An understudied class of proteins in phosphotyrosine signaling, the receptor protein tyrosine phosphatases (RPTPs), are a family of single-pass transmembrane proteins whose architecture include an extracellular domain resembling those of cell adhesion molecules (CAMs) and intracellular single or tandem tyrosine phosphatase domains. In vertebrates, this diversity is typified by the leukocyte common antigen related (Lar) and its two homologs RPTPδ/PTPRD and RPTPσ/PTPRS, which form the type IIa family of RPTPs. The ectodomains of Lar-RPTPs resemble immunoglobulin (Ig)-superfamily CAMs and include three Ig-like domains followed by four to nine fibronectin type III (FN) repeats. Surprisingly, we uncovered a tripeptide, Lys-Gly-Asp (KGD), in the Dlar FN5 domain that is similar to the RGD motif in FN10 and is conserved in the Lar-RPTP homologs across species.

We sought to gain further insights into the position of the conserved KGD motif in mammalian homologues of Dlar. We thus determined the crystal structures of the FN5 domain of mouse LAR and the FN4-FN6 fragment of human RPTPδ. The LAR FN5 crystal structure was solved by molecular replacement using Dlar FN5 as the model and refined to a resolution of 1.7 Å, while the structure of the FN4-FN6 fragment was to a resolution of 1.77 Å. A similar conclusion can be drawn from examining the position of the KGD sequence within the structure of RPTPδ FN4-FN6. The three-domain fragment adopts an extended conformation, but the KGD sequence lies at the interface between domains FN4 and FN5, which makes the tripeptide unavailable for binding to integrins. Thus, if Dlar and its mammalian homologues interact directly with integrins, they will use a mechanism that is distinct from the canonical RGD/integrin binding interaction. (D) The crystal structure of domains FN4-FN6 of human RPTPδ is shown in a ribbon representation and colored green. The lysine and aspartate residues found in the KGD motif are shown in ball-and-stick representation.

> PSTGSKPSAPPQDISCTSPSSTSILVSWQPPPVEKQNGIITEYSIKYTAVDGEDDKPHEILGIPSDTTKYLLEQLEKWTEYRITVTAHTDVGPGPESLSVLIRTNEDVPSGPPRKVEVEAVNSTSVKVSWRSPVPNKQHGQIRGYQVHYVRMENGEPKGQPMLKDVMLADAQWEFDDTTEHDMIISGLQPETSYSLTVTAYTTKGDGARSKPKLVSTTGAVPGKPRLVINHTQMNTALIQWHPPVDTFGPLQGYRLKFGRKDMEPLTTLEFSEKEDHFTATDIHKGASYVFRLSARNKVGFGEEMVKEISIPEE> MNLSLSDLHRQVSRLVQQESGDCTGK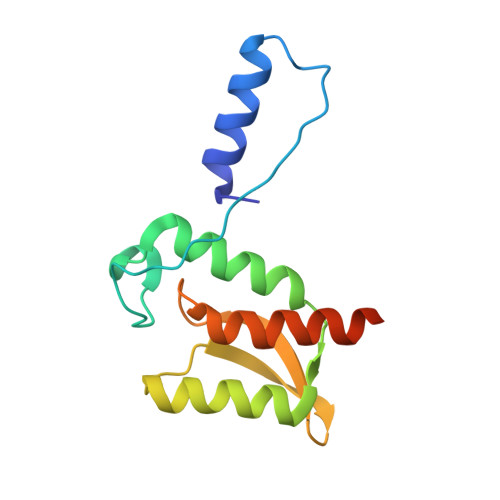LRGNVAANKETTFQGLTIASGARESEKVFAQTVLSHVANVVLTQEDTAKLLQSTVKHNLNNYDLRSVGNGNSVLVSLRSDQMTLQDAKVLLEAALRQESGARGSHHHHHH> 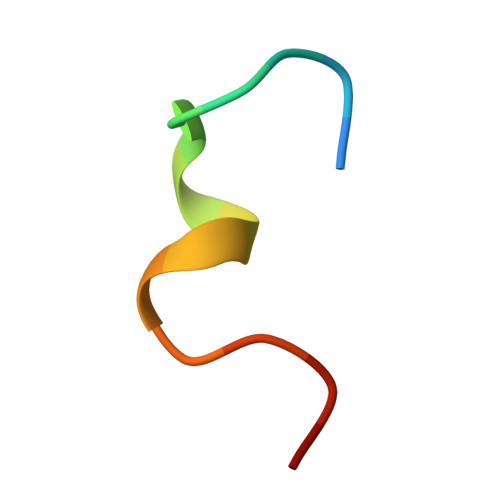XYDYPGDFCYLYGTCX>MLKKNDIVEVEIVDLTHEGAGVAKVDGLVFFVENALPSEKILMRVLKVNKKIGFGKVEKYLVQSPHRNQDLDLAYLRSGIADLGHLSYPEQLKFKTKQVKDSLYKIAGIADVEVAETLGMEHPVKYRNKAQVPVRRVNGVLETGFFRKNSHNLMPLEDFFIQDPVIDQVVVALRDLLRRFDLKPYDEKEQSGLIRNLVVRRGHYSGQIMVVLVTTRPKVFRVDQLIEQVIKQFPEIVSVMQNINDQNTNAIFGKEWRTLYGQDYITDQMLGNDFQIAGP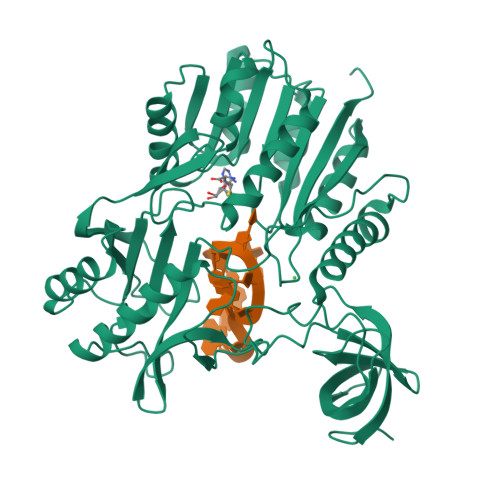AFYQVNTEMAEKLYQTAIDFAELKKDDVIIDAYSGIGTIGLSVAKHVKEVYGVELIPEAVENSQKNASLNKITNAHYVCDTAENAMKKWLKEGIQPTVILVDPPRKGLTESFIKASAQTGADRIAYISCNVATMARDIKLYQELGYELKKVQPVDLFPQTHHVQTVALLSKLDVD[2x]Obscurin, or its homolog obscurin-like-1, bridges the giant ruler titin and the myosin crosslinker myomesin at the M-band. Myomesin is a 185 kDa modular protein that localizes exclusively at the M-band, where anti-parallel dimers cross link myosin filaments. In addition to a mechanical role, myomesin is also needed for the integration of obscurin and its smaller obscurin-like-1 homolog at the M-band (Fukuzawa et al., 2008). Yeast two-hybrid and biochemical analyses have mapped the obscurin/obscurin-like-1:myomesin interaction to the linker region (L) located between the fourth and fifth Fn-III domains of myomesin (My4 and My5, respectively) and the third Ig domain of either obscurin or obscurin-like-1 (O3 and OL3, respectively) (inset) (Fukuzawa et al., 2008).

The ability of OL3:My4L to transition from the solution conformation to that observed crystallographically suggests that the LH helix might have a degree of flexibility. We explored this by solving the crystal structure of My4LH (myomesin residues 510–618) in two different space groups (data collection and refinement statistics in Table 1). In space group P65 (2.05 Å resolution), all four My4LH independent molecules in the a.u. display clear electron density until residue A608, while residues E609-S618 (LH) cannot be modeled. The same applies for four of six My4LH independent molecules in the alternative P21 space group (2.80 Å resolution). However, in the latter crystal structure, crystal contacts stabilize the C-terminal region in the remaining two other My4LH molecules. While in one molecule, LH folds into an α-helix as in the My4L:OL3 complex, in the other molecule the C-terminus is in a more extended conformation. Overall, SAXS and crystallographic analyses support a model in which interdomain freedom allows the transition from a relatively compact solution conformation to an open one that can be stabilized by homodimerization.

>[6x]GSTPAAPLDVKCLEANKDYIIISWKQPAVDGGSPILGYFIDKCEVGTDSWSQCNDTPVKFARFPVTGLIEGRSYIFRVRAVNKMGIGFPSRVSEPVAALDPAEKARLKSRPS>[2x]GHM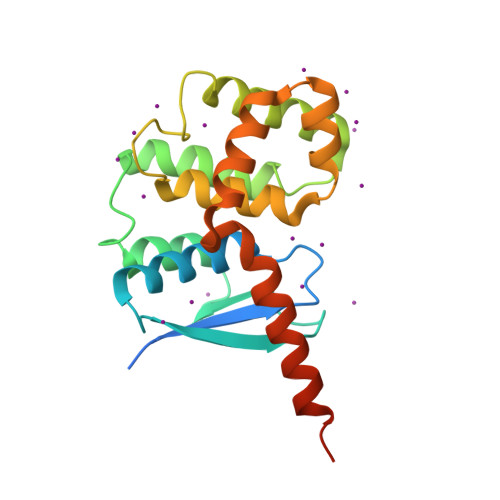TKLFSKVKESIEGIKMPSTLTINGKAPIVAYAELIAARIVNALAPNSIAIKLVDDKKAPAAKLDDATEDVFNKITSKFAAIFDNGDKEQVAKWVNLAQKELVIKNFAKLSQSLETLDSQLNLRTFILGGLKYSAADVACWGALRSNGMCGSIIKNKVDVNVSRWYTLLEMDPIFGEAHDFLSKSLLELKKSANVGKKKETHKANFE1-(2-hydroxyethyl)-5-[(4-methoxynaphthalen-1-yl)methyl]-~{N}-(phenylmethyl)-6,7-dihydro-4~{H}-pyrazolo[4,3-c]pyridine-3-carboxamide 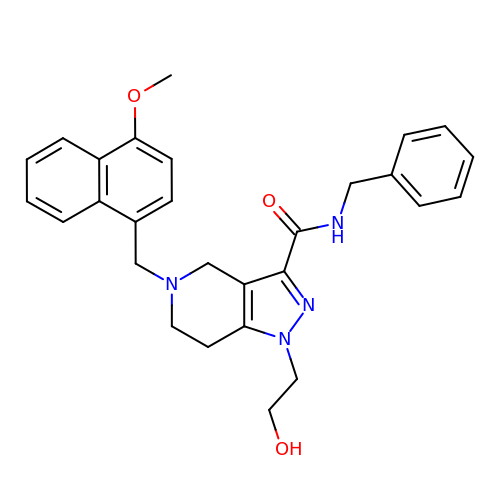| C28 H30 N4 O3 | ZHTGDAFDEHXYSS-UHFFFAOYSA-N>[12x]MGKYQVMKRASEVDLSTVKYKAETMKAPHLTGLSFKLFVNLLEAPLIGSLIVDYLKKDNGMTKIFRNTVIPEEPMFRPEFPSQEPEHDVVIVGEDESPIDRLETALKCLPQYDPSRSLHADPVSSFRYWKIRDYAYAYRSKLTTPLQVAKRIISIIEEFGYDKPPTPFLIRFDANEVIKQAEASTRRFEQGNPISVLDGIFVTIKDDIDCLPHPTN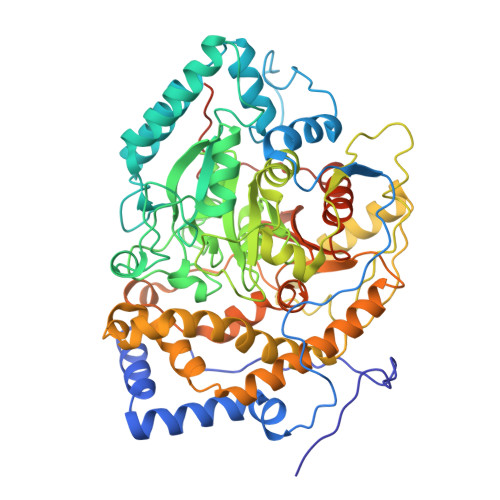GGTTWLHEDRSVEKDSAVVSKLRSCGAILLGKANMHELGMGTTGNNSNYGTTRNPHDPKRYTGGSSSGSAAIVAAGLCSAALGTDGGGAVRIPSALCGITGLKTTYGRTDMTGSLCEGGTVEIIGPLASSLEDAFLVYAAILGSSSADRYNLKPSPPCFPKLLSHNGSNAIGSLRLGKYTKWFNDVSSSDISDKCEDILKLLSNNHGCKVVEIVVPELEEMRAAHVISIGSPTLSSLTPYCEAGKNSKLSYDTRTSFAIFRSFSASDYIAAQCLRRRLMEYHLNIFKDVDVIVTPTTGMTAPVIPPDALKNGETNIQVTTDLMRFVLAANLLGFPAISVPVGYDKEGLPIGLQIMGRPWAEATVLGLAAAVEELAPVTKKPAIFYDILNTNKGEFEAYVEQKLISEEDLNSAVDHHHHHH[[(2~{R},3~{S},4~{R},5~{R})-5-[2,4-bis(oxidanylidene)pyrimidin-1-yl]-3,4-bis(oxidanyl)oxolan-2-yl]methoxy-oxidanyl-phosphoryl] propyl hydrogen phosphate | C12 H20 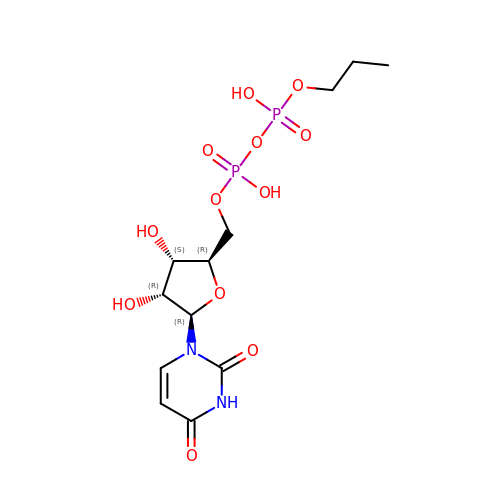N2 O12 P2 | INDMXLOHISKOMT-QCNRFFRDSA-N> APAAVDWRARGAVTAVKDQGQCGSCWAFSAIGNVECQWFLAGHPLTNLAEQMLVSCDKTDSGCSGGLMNNAFEWIVQENNGAVYTEDSYPYASGEGISPPCTTSGHTVGATITGHVELPQDEAQIAAWLAVNGPVAVAVDASSWMTYTGGVMTSCVSEQLDHGVLLVGYNDGAAVPYWI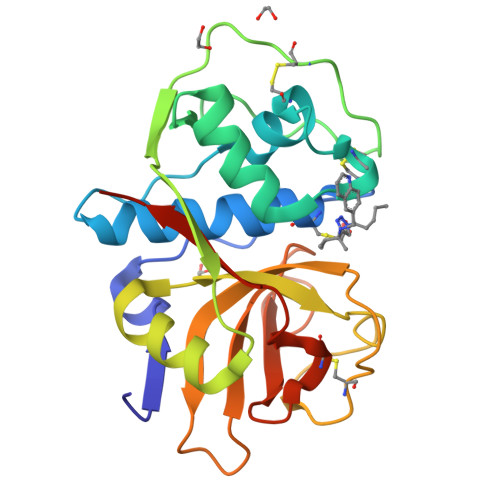IKNSWTTQWGEEGYIRIAKGSNQCLVKEEASSAVVGHHHHHH> AAHHRMRWRADGRSLEKLPVHMGLVITEVEQEPSFSDIASLVVWCMAVGISYISVYDHQGIFKRNNSRLMDEILKQQQELLGLDCSKYSPEFANSNDKDDQVLNCHLAVKVLSPEDGKADIVRAAQDFCQLVAQKQKRPTDLDVDTLASLLSSNGCPDPDLVLKFGPVD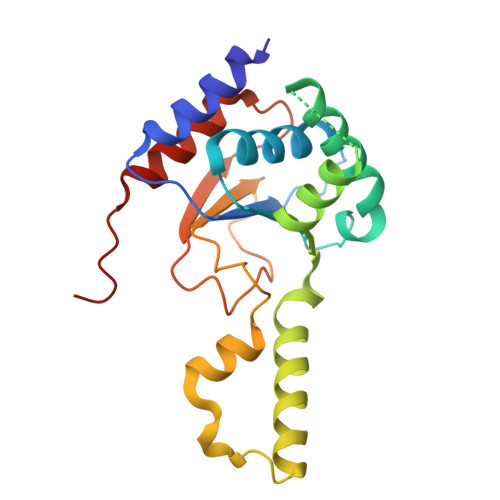STLGFLPWHIRLTEIVSLPSHLNISYEDFFSALRQYAACEQRLGK> IGDEPLENYLDTEYFGTIGIGTPAQDFTVIFDTGSSNLWVPSVYCSSLACSDHNQFNPDDSS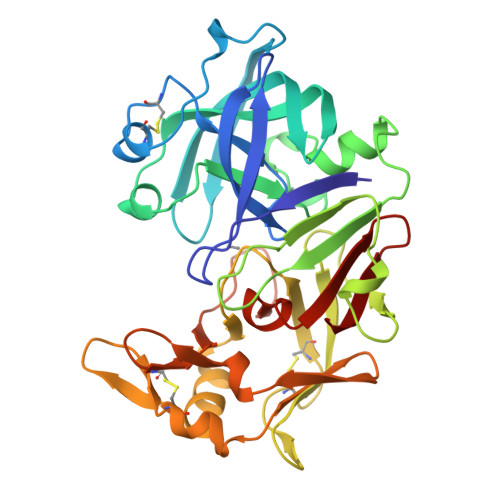TFEATSQELSITYGTGSMTGILGYDTVQVGGISDTNQIFGLSETEPGSFLYYAPFDGILGLAYPSISASGATPVFDNLWDQGLVSQDLFSVYLSSNDDSGSVVLLGGIDSSYYTGSLNWVPVSVEGYWQITLDSITMDGETIACSGGCQAIVDTGTSLLTGPTSAIANIQSDIGASENSDGEMVISCSSIDSLPDIVFTIDGVQYPLSPSAYILQDDDSCTSGFEGMDVPTSSGELWILGDVFIRQYYTVFDRANNKVGLAPVA>[7x]GSMSAEGYQYRALYDYKKEREEDIDLHLGDILTVNKGSLVALGFSDGQEAKPEEIG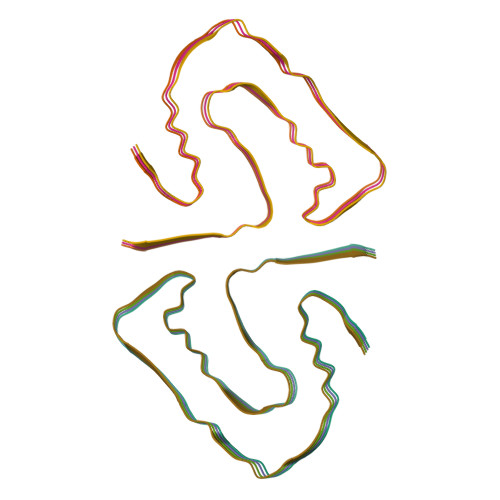WLNGYNETTGERGDFPGTYVEYIGRKKISP>GENSDNLTHCRLFEFRLCLLECMSLTLDHCYARCTTVITQIHGSDTNRFDCTIFKTCYYRCYVLGKTEDHCWKGTATSVTGDVGDLEFC[6x]

The venoms of marine cone snails constitute a particularly rich source of peptide toxins, known as conotoxins. Here, we identify the sequence of an unusually large conotoxin, Mu8.1, which defines a new class of conotoxins evolutionarily related to the well-known con-ikot-ikots and 2 additional conotoxin classes not previously described. The crystal structure of recombinant Mu8.1 displays a saposin-like fold and shows structural similarity with con-ikot-ikot. Functional studies demonstrate that Mu8.1 curtails calcium influx in defined classes of murine somatosensory dorsal root ganglion (DRG) neurons. When tested on a variety of recombinantly expressed voltage-gated ion channels, Mu8.1 displayed the highest potency against the R-type (Cav2.3) calcium channel.

To elucidate key structural features of the SLC superfamily, we determined crystal structures of Mu8.1 from 2 different crystal conditions referred to as Mu8.1_38 and 59 at resolutions of 2.33 Å and 2.1 Å, respectively. The asymmetric unit of Mu8.1_59 accommodates 6 molecules that form 3 equivalent dimers. Each protomer of the Mu8.1 structure comprises 2 regions. The first region comprises an N-terminal 310-helix (310N), followed by 2 α-helices (α1 and α2), and a 310-linker helix (310L). The second region comprises 2 α-helices (α3 and α4), and the C-terminal 310-helix (310C). The 2 helical regions surround a hydrophobic core predominantly formed by aromatic residues (Phe15, Tyr31, Tyr58, Tyr59, Trp72). Moreover, α1, α3, and α4 are held together by a network of contacts between Arg16, Tyr58, Glu68, and Trp72, where ionic interactions are present between the side chains of Arg16 and Glu68, whereas Tyr58 and Trp72 partake in T-shaped pi–pi interactions. The dimer interface is characterized by both hydrophobicity as well as the presence of a water-filled cavity surrounded by the polar residues Thr36, Asn47, Thr52, and Thr56. The residues forming the largely dry (water-excluded) hydrophobic interface include Tyr31, Ala32, Phe49, Ile53, Tyr59, and Val83. Based on evidence from the analytic gel filtration and SAXS measurements, we concluded that Mu8.1 exists primarily as a dimer in solution.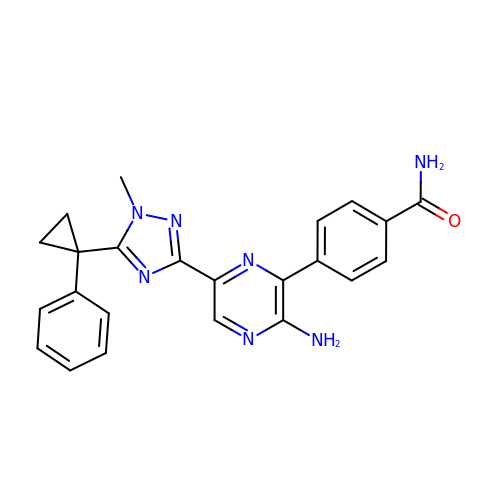4-[3-azanyl-6-[1-methyl-5-(1-phenylcyclopropyl)-1,2,4-triazol-3-yl]pyrazin-2-yl]benzamide | C23 H21 N7 O | OASVVQQPBXNNOH-UHFFFAOYSA-N>[2x]MFIRIKCFSKQPIAKKVSREVSAYLEYTGNNTWEGHISGQGVSNLQTKLINVGKGVKVVCNYQDKVLFAIGNVAMSDTGSVPKY;>MQKQILTSQKRNMYILSRCKVLVKNGQVCHLHEDGNVYTVPYANTVFIGLAEGTSITNEAMSMLAANGVIVFWTKGGGYDMFAADIICHLPQADYRPTKYMQNWVRLWLDEEKKLSAAKEI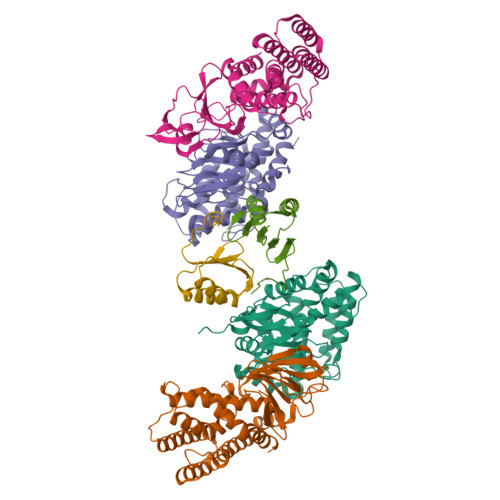LKMRVDSLSTHVHDFGVDVENKRVSSIVNKFDKGVTQATSFESLLGHEGTFVKSLYKEYALEYEIEFKRDHKSADNYNKFLTLGNYYAYGIARSSLWALGIDNSFPLLHGSTRRGGLVFDVADIIKTSIILPLAFHAADQGMSNTEFKRSCVAYFDKNDILAYLINNIKRLCMEN[4x]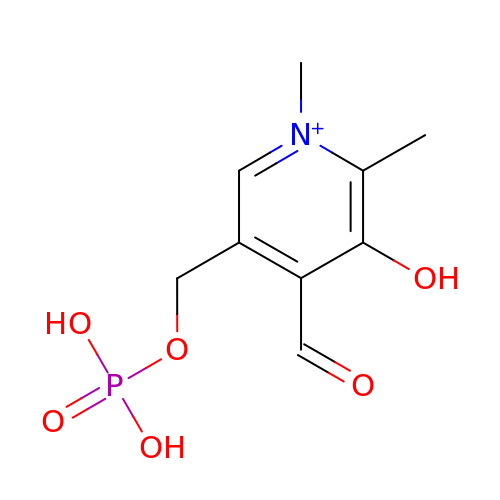N-METHYL-PYRIDOXAL-5'-PHOSPHATE | C9 H13 N O6 P | CBNMAKRKGWDQHB-UHFFFAOYSA-O> ALDFSKWKTRQPGEFRAPCPAMNSLANHGFIPRDGRNITVAMLVPVLQEVFHLSPELAQTISTLGLFTAQDPSKGVFTLDDLNRHNLFEHDASLSREDYY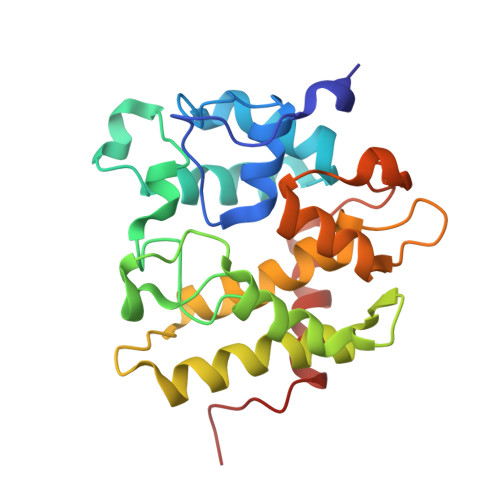FHKDASTFRPEVFKKFMSHFKGKEYVTLEDAASARYAMVQESRKKNPTFTYTVQQRITSYGETIKYFRTIVEPATGKCPVAWIKILFEQERLPYNEGWRPPKAELSGFSMASDVLELALVTPEKLID> GHMEELNIDFDVFKKRIELLYSKYNEFEGSPNSLLFVLGSSNAENPYQKTTILHNWLLSYEFPATLIALVPGKVIIITSSAKAKHLQKAIDLFKDPESKITLELWQRNNKEPELNKKLF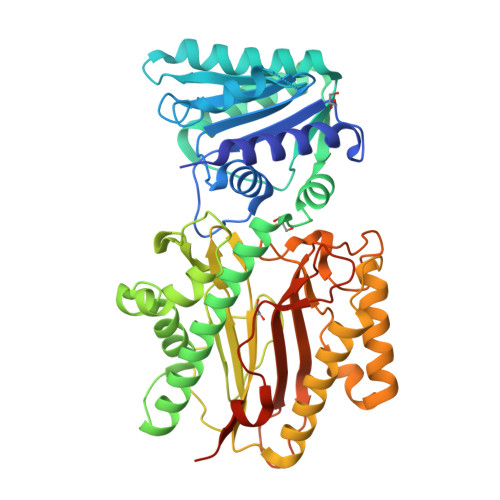DDVIALINSAGKTVGIPEKDSYQGKFMTEWNPVWEAAVKENEFNVIDISLGLSKVWEVKDVNEQAFLSVSSKGSDKFMDLLSNEMVRAVDEELKITNAKLSDKIENKIDDVKFLKQLSPDLSALCPPNYKFNFDLLDWTYSPIIQSGKKFDLRVSARSTNDQLYGNGCILASCGIRYNNYCSNITRTFLIDPSEEMANNYDFLLTLQKEIVTNILKPGRTPKEVYESVIEYIEKTKPELVPNFTKNIGSLIGLEFRDSNFILNVKNDYRKIQRGDCFNISFGFNNLKDSQSANNYALQLADTVQIPLDETEPPRFLTNYTKAKSQISFYFNNEEEDNNKKKSSPATKV> YEETPDVIGKSVKEAEQIFNKNNLKLGKISRSYSDKYPENEIIKTTPNTGERVERGDSVDVVISKGPEKVKMPNVIGLPKEEALQKLKSLGLKDVTIEKVYNNQAPKGYIANQSVTANTEIAIHDSNIKLYESLGIKQVYVEDFEHKSFSKAKKALEEKGFKVESKEEYS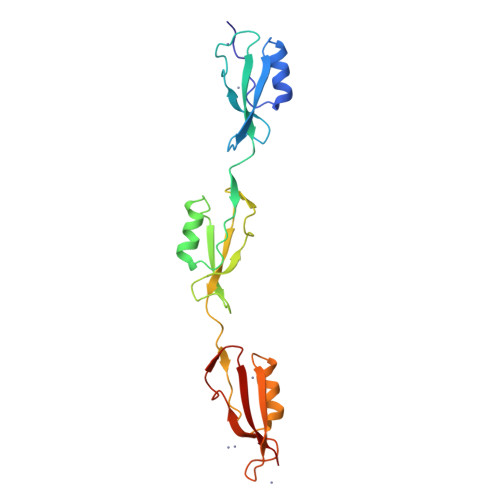DDIDEGDVISQSPKGKSVDEGSTISFVVSKG>MSSAIKEVQGAPVKWVTNWTPEAIRGLVDQEKGLLDPRIYADQSLYELELERVFGRSWLLLGHESHVPETGDFLATYMGEDPVVMVRQKDKSIKVFLNQCRHRGMRICRSDAGNAKAFTCSYHGWAYDIAGKLVNVPFEKEAFCDKKEGDCGFDKAEWGPLQARVATYKGLVFANWDVQAPDLETYLGDARPYMDVMLDRTPAGTVAIGGMQKWVIPCNWKFAAEQFCSDMYHAGTTTHLSGILAGIPPEMDLSQAQIPTKGNQFRAAWGGHGSGWYVDEPGSLLAVMGPKVTQYWTEGPAAELAEQRLGHTGMPVRRMVGQHMTIFPTCSFLPGINTIRTWHPRGPNEIEVWAFTLVDADAPAEIKEEYRRHNIRNFSAGGVFEQDDGENWVEIQKGLRGYKAKSQPLNAQMGLGRSQTGHPDFPGNVGYVYAEEAARGMYHHWMRMMSEPSWATLKP[12x];>[12x]MTNPSPHFFKTFEWPSKAAGLELQNEIEQFYYREAQLLDHRAYEAWFALLDKDIHYFMPLRTNRMIREGELEYSGDQDLAHFDETHETMYGRIRKVTSDVGWAENPPSRTR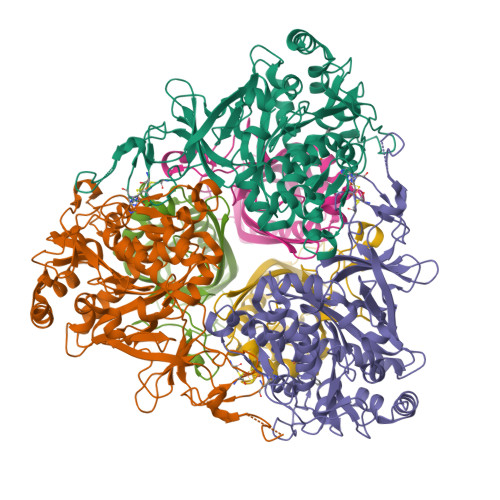HLVSNVIVKETATPDTFEVNSAFILYRNRLERQVDIFAGERRDVLRRADNNLGFSIAKRTILLDASTLLSNNLSMFF> MGQEGKGTCILVGGHEITSGLEVISSLRAIHGLQVEVCPLNGCDYIVSNRMVVERRSQSEMLNSVNKNKFIEQIQHLQSMFERICVIVEKDREKTGDTSRMFRRTKSYDSLLTTLIGAGIRILFSSCQEETADLLKELSLVEQRKNVGIH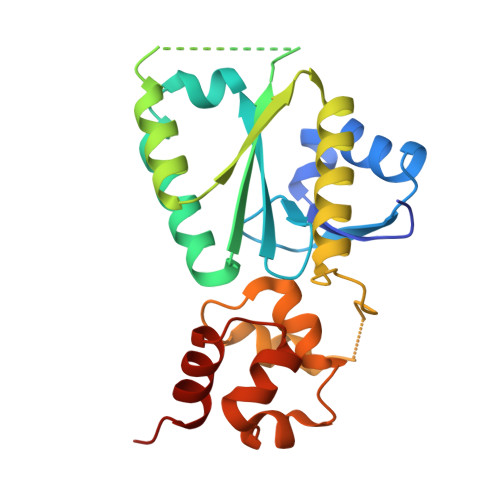VPTVVNSNKSEALQFYLSIPNISYITALNMCHQFSSVKRMANSSLQEISMYAQVTHQKAEEIYRYIHYVFD>[2x]MSLKIKNILLS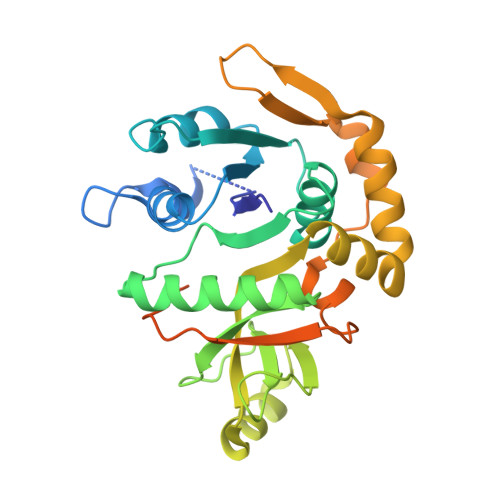GGSGKRLWPLSRSLYPKQFLKLFDHKSLFELSFKRNASLVDETLIVCNEKHYFLALEEIKNEIKNKSVGFLLESLSKNTANAIALSALMSDKEDLLIVTPSDHLIKDLQAYENAIKKAIDLAQKGFLVTFGVSIDKPNTEFGYIESPNGLDVKRFIEKPSLDKAIEFQKSGGFYFNSGMFVFQAGVFLDELKKHAPTILKGCERAFESLENAYFFEKKIARLSEKSMQDLEDMSIDIALMQQSHKIKMVELNAKWSDLGNFNALFEEAANEPKENVSLNQTPVFAKESEEGHHHHHH> GNKTGITYPEIKLGETGKDIKTTITFMNNRTDMNLDTYPGKNWKSYIEDFNKMYPNITVKVQTDSNYADSALTRLQANNDSWDIMMIPAVDKSEFSNYFVPYGETSEMEKVIKLADEKAYDGQTYGIANNGVTAGIVYNKKVFEEAGIKELPKT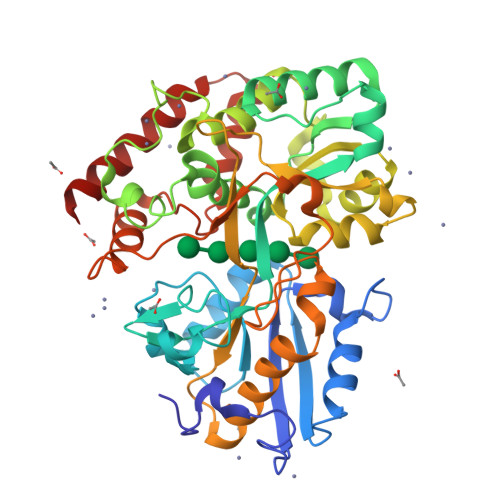PEEFQADLKLIKEKTKAVPLYTNFVEDWAMGAWDQYIAGNATGDPKFMNQVLPTTKEPFKKDASAPDTHPYAVYKTLYDAVANGYTEEDYSTTDWESSKGKMNNGEIATMVLGAWAVPQMKQAGDHPDDIGYMPFPITVDGKQYATIAGDYSYGINKNISKEKQEASMIFVKWMTEDSGFAKNEGGIPIKADDESMPETYETFSDVELITDAPAKEGQEDLLANVNSDSELGINNGNGKKIQDIVVDAANRTRTIDQIMDEWNQKWAKAVEDN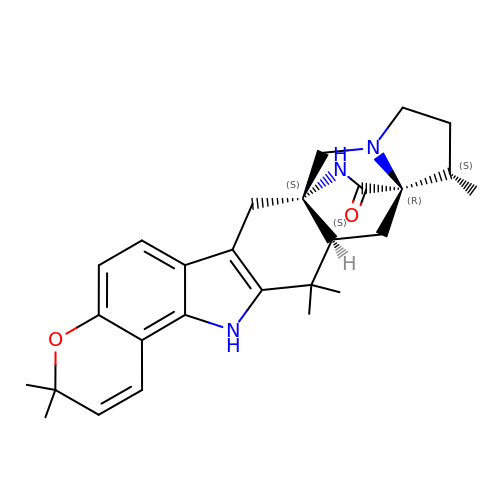(7aS,12S,12aR,13aS)-3,3,12,14,14-pentamethyl-3,7,11,12,13,13a,14,15-octahydro-8H,10H-7a,12a-(epiminomethano)indolizino[6,7-h]pyrano[3,2-a]carbazol-16-one | C27 H33 N3 O2 | NZXZONUAPKPCQR-CVXXBLRVSA-N>GPMAKVKKHLTFSGPTESPYGIAYIEKEMKAKNCSKMNETIELIFAEHDEMKARLSEQDALVEKIFQRFKKTLDVIRVR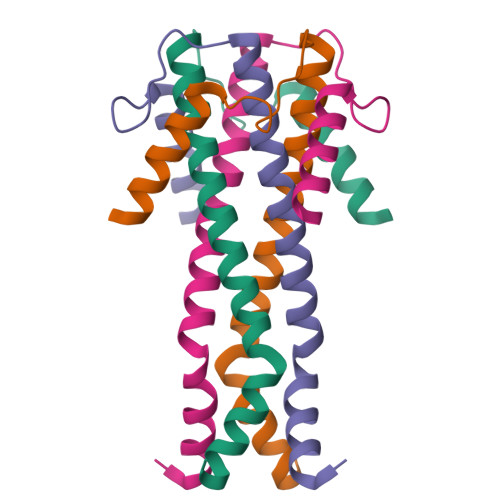AGHTDKNAQINLELWNAFLMANPLPVTVLTDQHTSESVSMAKEKVSNDIATFKQRKDEQKAKQEMQKGEK[2x]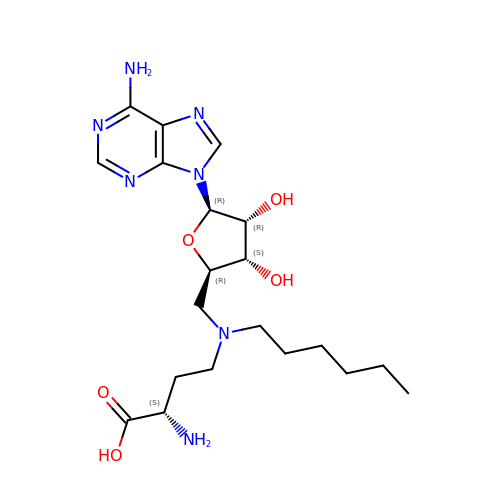5'-{[(3S)-3-amino-3-carboxypropyl](hexyl)amino}-5'-deoxyadenosine | C20 H33 N7 O5 | PUFLVFWUSGLSNL-BPAMBQHCSA-N>[2x]GSKLETKQRSPVEIIDDVKDEIQKRELIYDALHKLNSPNEEKEYFNIHAWDVWHDMISVRALTVDSDVEIYKVLKAMSSAKITQATTGYKGTQLKAMFSLDGPQIQNVVFKPKRYSRNKIILGTP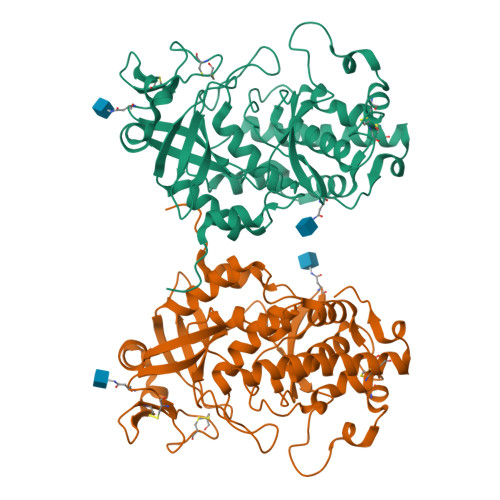YEGYDRHNAEIAAFHLDRLLGFYRAPPVVGRYINLAAEVLPVAAKKLATTFIKDKDENLCFYGKCLYCNRKEPACASNVTMEGALILWLPEKWPVLKLPHPWRRTYNKKMAKWETDSHYCESVVIKEPYTKGPRLLDLIDTSIFDFLIGNADRHHYEYIENENGSMVIHLDNAKSFGNPFVDEKSILSPLVQCCRLRSSTYNRLKIATSNENSLSVLLDKRLSIDPIYPILTSDHLLALDRRLLLVQDAVEKCFKEKNKENVIIEDHL>[2x]ARIRAPQEATVKEVHDAPAVRGSIIANMLQEHDNPFTLYPYDTNYLIYTQTSDLNKEAIASYDWAENARKDEVKFQLSLAFPLWRGILGPNSVLGASYTQKSWWQLSNSEESSPFRETNYEPQLFLGFATDYRFAGWTLRDVEMGYNHDSNGRSDPTSRSWN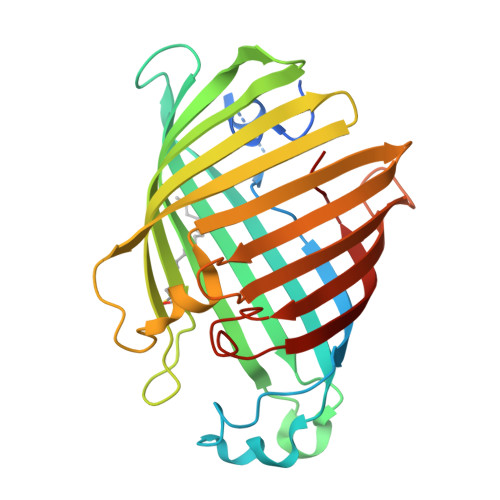RLYTRLMAENGNWLVEVKPWYVVGNTDDNPDITKYMGYYQLKIGYHLGDAVLSAKGQYNWNTGYGGAELGLSYPITKHVRLYTQVYSGYGESLIDYNFNQTRVGVGVMLNDLF> MTTRMIILNGGSSAGKSGIVRCLQSVLPEPWLAFGVDSLIEAMPLKMQSAEGGIEFDADGGVSIGPEFRALEGAWAEGVVAMARAGARIIIDDVFLGGAAAQERWRSFVGDLDVLWVGVRCDGAVAEGRET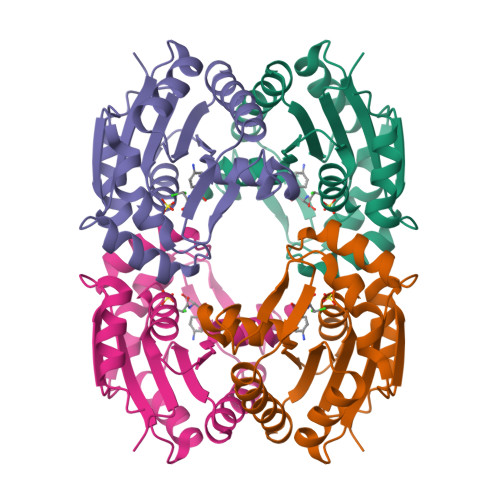ARGDRVAGMAAKQAYVVHEGVEYDVEVDTTHKESIECAWAIAAHVVP> MSDKTKTNEGFSRRSFIGSAAVVTAGVAGLGAIDAASATQKTNRASTVKGGFDYDVVVVGGGFAGATAARECGLQGYRTLLLEARSRLGGRTFTSRFAGQEIEFGGAWVHWLQPHVWAEMQRYGLGVVEDPLTNLDKTLIMYNDGSVESISPDEFGKNIRIAFEKLCHDAWEVFPRPHEPMFTERARELDKSSVLDRIKTLGLSRLQQAQINSYMALYAGETTDKFGLPGVLKLFACGGWNYDAFMDTETHYRIQGGTIGLINAMLTDSGAEVRMSVPVTAVEQVNGGVKIKTDDDEIITAGVVVMTVPLNTYKHIGFTPALSKGKQRFIKEGQLSKGAKLYVHVKQNLGRVFAFADEQQPLNWVQTHDYSDELGTILSITIARKETIDVNDRDAVTREVQKMFPGVEVLGTAAYDWTADPFSLGAYAAYGVGQLSRLKDLQAAEGRILFAGAETSNGWHAYIDGAVESGLRAGREVKQLLSLEHH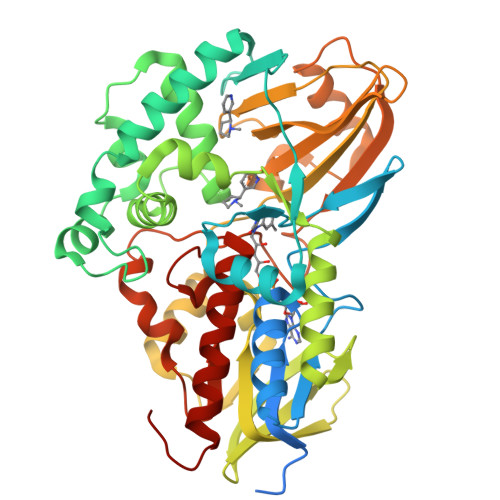HHHH> MHHHHHHENLYFQSDAICIYLDESATWKDMKKAMEILYKLGVKKIVVLFKYDEKLIKVAAKVLHDLGAEEAIIILIFDIDDEDEFKKQVKKALELMKKLGVDHRIIALRMTDEEKFKKLAKIAAELGADAICIYLDESATWKDMKKAMEILYKLGVKKIVVLFKYDEKLIKVAAKVLHDLGAEEAIIILIFDIDDEDEFKK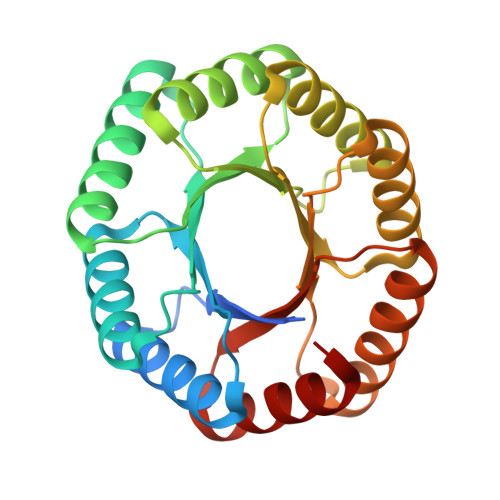QVKKALELMKKLGVDHRIIALRMTDEEKFKKLAKIAAELGA>DDNSAITKANGENNAVVKINKTLNIAEGITTPTATFTFKFTEKTGQSSNGAPYQTGVAIPDRNVEYNKNDHPTADKIQKATEDIFSGVAYGHAGEYVYDVAEAKTGWQAITKNG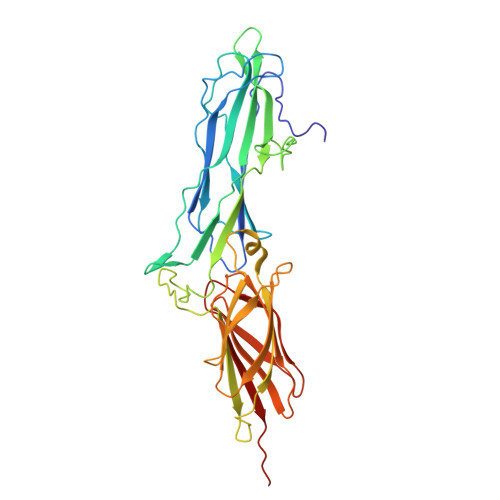KTIDAMRYDKRTYEMHVIVKNKVNGGVYISSVYFKENNKSNAPKVESSEQGVYNLFDNTYTKDASKEPNPDDPSQVDPNAKALTITKKVDGASGDKTRDFQFHIKIQLPSTNKTAETPVTNIIVKHGSKSEVLAVVTPADTVEYNFTLKDGETFTVEQLPAGSKYTVTETGVAGYTDSSIYTTNGAEQTSQGQKNVDFTLTDILIGEKKNDNKVTNKIDDVTPTGLL[2x]>[2x]ATTYNAVVSKSSSDGKTFKTIADAIASAPAGSTPFVILIKNGVYNERLTITRNNLHLKGESRNGAVIAAATAAGTLKSDGSKWGTAGSSTITISAKDFSAQSLTIRNDFDFPANQAKSDSDSSKIKDTQAVALYVTKSGDRAYFKDVSLVGYQDTLYVSGGRSFFSDCRISGTVDFIFGDGTALFNNCDLVSRYRADVKSGNVSG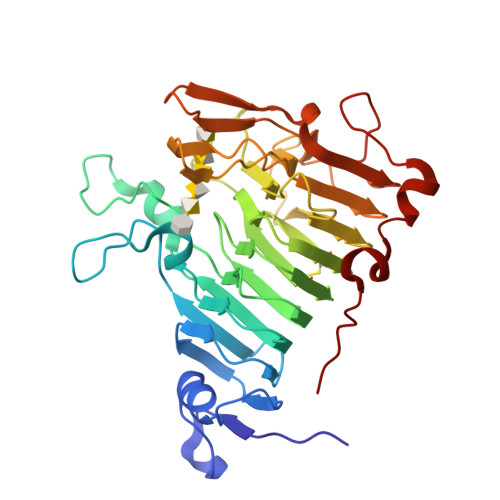YLTAPSTNINQKYGLVITNSRVIRESDSVPAKSYGLGRPWHPTTTFSDGRYADPNAIGQTVFLNTSMDNHIYGWDKMSGKDKNGNTIWFNPEDSRFFEYKSYGAGATVSKDRRQLTDAQAAEYTQSKVLGDWTPTLP The tripartite motif (TRIM) proteins form one of the largest subfamilies of RING-type E3 ubiquitin ligases, comprising more than 80 members. TRIM family members typically contain a RING domain usually catalyzing ubiquitin transfer; one or two B-box domains mediating protein–protein interactions; and a large coiled-coil domain region, which is involved in self-association or oligomerization with other TRIM E3-ligase proteins (Fiorentini et al., 2020, Ozato et al., 2008). About two-thirds of human TRIM proteins feature a PRYSPRY domain, also known as the B30.2 domain, in their C-terminal region. All characterized family members shared the same overall PRYSPRY twisted β-sandwich fold consisting of a 7-stranded and a 6-stranded antiparallel β-sheet.

A characteristic feature of the putative substrate-binding site in the closely related homologs MID1 and MID2 is an arginine located at the C-terminus of β-strand 7 (R587 in MID1 and R637 in MID2) that projects its guanidinium group toward the center of the cavity and two neighboring tryptophan residues lining the pocket. The orientation of the side chain of the two tryptophan residues in MID2, Trp602 and Trp694, showed an intriguing variation in the crystal structures. The MID2 domain was solved in two different crystal forms. In the C2221 crystal form, which contains one protein molecule per asymmetric unit, the side chains of Trp602 and Trp694 engage in π-stacking interactions.

> SMNSQPFKLDPKMTHKKLKISNDGLQMEKDESSLKKSHTPERFSGTGCYGAAGNIFIDSGCHYWEVVMGSSTWYAIGIAYKSAPKNEWIGKNASSWVFSRCNSNFVVRHNNKEMLVDVPPHLKRLGVLLDYDNNMLSFYDPANSLHLHTFDVTFILPVCPTFTIWNKSLMILSGLPAPDFIDYPERQECN> 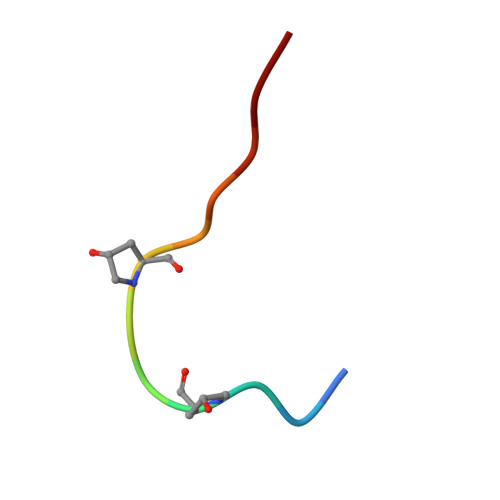RLVPSGPNPLHN>SDTECHFCKSVINQAWNTSEQAMPQAMHQACLRFWLDRQKCEQFVEQHMPQLLALVPRSQDAHITC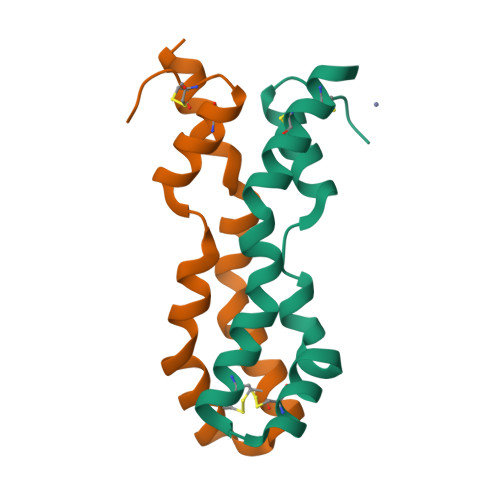QALGVCEAPAS[2x]>[2x]HHHHHHSSGLVPRGSHMISHIGTIDVFVNDQDKAIDFYVNTLGFELREDQAFGPMRWVEVAPAGSQTRIVLCTKHFPVYEEGKIGRFTDIQLVTEDIKATHEE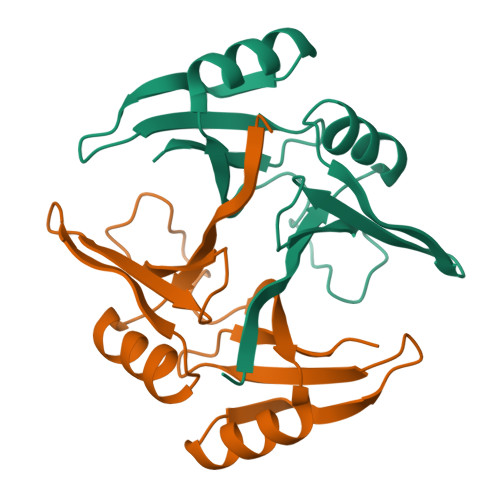LVRRGVNFTRAPEQMPFGGANASFQDPDGNEFLLLQPSR>[4x]ADDAKPRVKVPSSAKAGETVTVKALISHKMESGQRK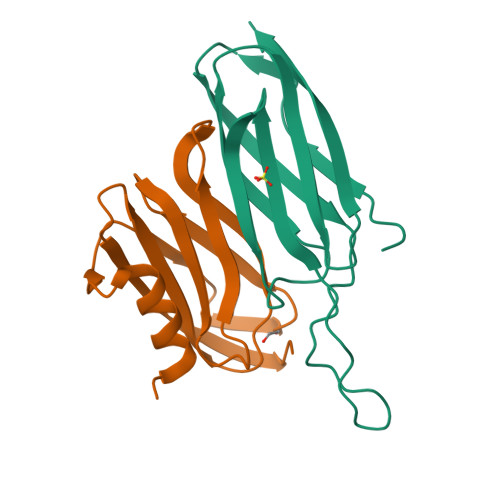DADGKLIPRSIINRFTCELNGVNVVDVAIDPAVSTNPYFEFDAKVDAAGEFKFTWYDDDGSVYEDVKPIAVA;>[4x]MRGSHHHHHHGSSTVDELTAAFTGGAATGEGGLTLTAPEIAENGNTVPIEVKAPGAVAIMLLAAGNPEPAVATFNFGPAAADQRAATRIRLAQTQDVIALAKMADGSVVKAQTTVKVTIGGCGG> TAPQWV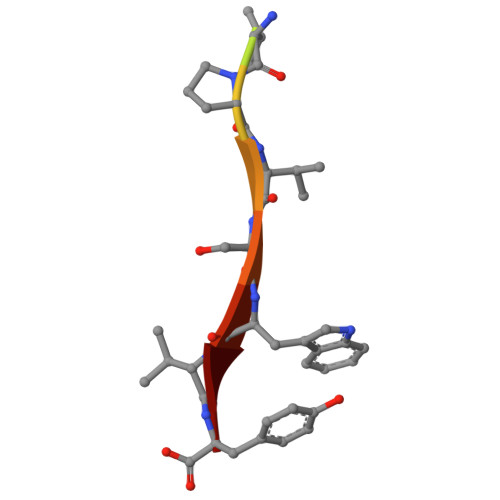PVSWVY>[2x]MTGMSREEVESLIQEVLEVYPEKARKDRNKHLAVNDPAVTQSKKCIISNKKSQPGLMTIRGCAYAGSKGVVWGPIKDMIHISHGPVGCGQYSRAGRRNYYIGTTGVNAFVTMNFTSDFQEKDIVFGGDKKLAKLIDEVETLFPLNKGISVQSECPIGLIGDDIESVSKVKGAELSKTIVPVRCEGFRGVSQSLGHHIANDAVRDWVLGKRDEDTTFASTPYDVAIIGDYNIGGDAWSSRILLEEMGLRCVAQWSGDGSISEIELTPKVKLNLVHCYRSMNYISRHMEEKYGIPWMEYNFFGPTKTIESLRAIAAKFDESIQKKCEEVIAKYKPEWEAVVAKYRPRLEGKRVMLYIGGLRPRHVIGAYEDLGMEVVGTGYEFAHNDDYDRTMKEMGDSTLLYDDVTGYEFEEFVKRIKPDLIGSGIKEKFIFQKMGIPFREMHSWDYSGPYHGFDGFAIFARDMDMTLNNPCWKKLQAPWEASEGAEKVAASA;>[2x]MSQQVDKIKASYPLFLDQDYKDMLAKKRDGFEEKYPQDKIDEVFQWTTTKEYQELNFQREALTVNPAKACQPLGAVLCALGFEKTMPYVHGSQGCVAYFRSYFNRHFREPVSCVS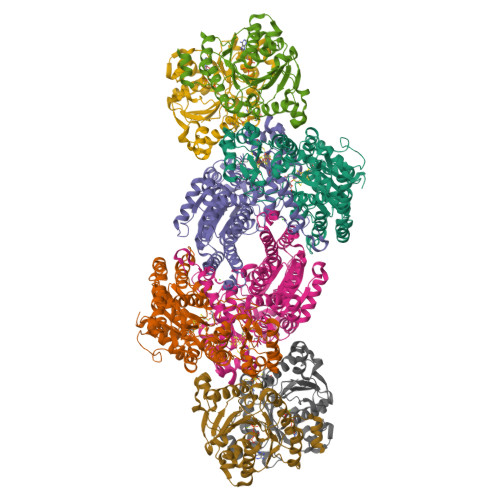DSMTEDAAVFGGQQNMKDGLQNCKATYKPDMIAVSTTCMAEVIGDDLNAFINNSKKEGFIPDEFPVPFAHTPSFVGSHVTGWDNMFEGIARYFTLKSMDDKVVGSNKKINIVPGFETYLGNFRVIKRMLSEMGVGYSLLSDPEEVLDTPADGQFRMYAGGTTQEEMKDAPNALNTVLLQPWHLEKTKKFVEGTWKHEVPKLNIPMGLDWTDEFLMKVSEISGQPIPASLTKERGRLVDMMTDSHTWLHGKRFALWGDPDFVMGLVKFLLELGCEPVHILCHNGNKRWKKAVDAILAASPYGKNATVYIGKDLWHLRSLVFTDKPDFMIGNSYGKFIQRDTLHKGKEFEVPLIRIGFPIFDRHHLHRSTTLGYEGAMQILTTLVNSILERLDEETRGMQATDYNHDLVR;>[4x]MAMRQCAIYGKGGIGKSTTTQNLVAALAEMGKKVMIVGCDPKADSTRLILHSKAQNTIMEMAAEAGTVEDLELEDVLKAGYGGVKCVESGGPEPGVGCAGRGVITAINFLEEEGAYEDDLDFVFYDVGDVVCGGFAMPIRENKAQEIYIVCSGEMMAMYAANNISKGIVKYANSGSVRLGGLICNSRNTDREDELIIALANKLGTQMIHFVPRDNVVQRAEIRRMTVIEYDPKAKQADEYRALARKVVDNKLLVIPNPITMDELEELLMEFGIMEVEDESIVGKTAEEV> SGTFFKDYQKKNVMRLLQDSLEKIINEWLKTDDESHTK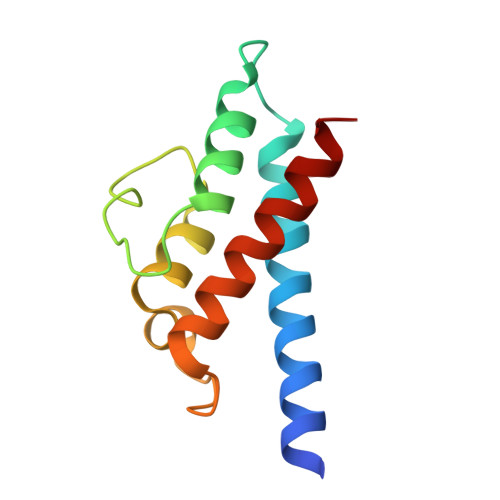LKSLQELSEMDINATSFAEHSPLPDFVTRLWLDPHKALDAMDKNISKNEIRKLIKETAREIELVFTH The modA/tupA/wtpA gene encodes a periplasmic molybdate/tungstate-binding protein (protein A) which constitutes the first selection gate from which cells should differentiate between Mo and W. The ModA, WtpA, and TupA proteins differ in their binding affinity for molybdate versus tungstate, primary sequence and oxoanion coordination chemistry. The present work reports the 1.40 Å crystal structure of the recombinant apo-form of TupA protein from the sulfate reducing bacteria Desulfovibro alaskensis G20 (DaG20 TupA) together with the biochemical characterization of three variants: R118K, R118E and R118Q. X-ray crystallography and SAXS, reveals that TupA architecture has a common feature with other substrate binding proteins, which is the existence of two separate lobes.

TupA is a globular protein with approximate dimensions of 55.7 × 34.5 × 23.8 Å. The protein has a butterfly shape with a central beta strand (T77-P89) that supports two lobes (lobe A: A2-R76 and Y201-E251; lobe B: A91-Q200). The central beta strand is hydrogen bonded to three beta strands of each of the lobes forming two 4-stranded beta sheets. The TupA metal binding site is located in a central cleft assembled by the two lobes. In DaG20 TupA, the cleft is decorated with positively charged residues as seen by the electrostatic surface potential calculations. The pronounced positive environment of the pocket must be an advantage to enable capture of the oxyanion, even when the extracellular concentration is low. Moreover, one chloride anion, arising from the crystallization conditions, was found at 3.8 Å from R118, indicating the propensity of the pocket to attract negatively charged ions. In this GsTupA-W6+ holo form, the central cleft volume (363.9 Å3) is four times smaller than the apo form of DaG20 TupA here reported (1480 Å3). The apo-form model was created by refining the initial BUNCH model with the SREFLEX program. This approach revealed a slight opening of the lobes (RMSD of 1.5 Å for 274 Cα atoms) yielding an excellent agreement to the TupA SAXS data measured in the absence of tungstate or molybdate (χ2 = 1.0). The SAXS data corroborate the hypothesis that DaG20 TupA is a flexible protein that is able to adopt a loose conformation in the free form but, when binding to molybdate or tungstate, switches to a more compact fold.

> MAHHHHHHVDDDDKMLEVLFQGPEAPVLMMATTTSTDNTGLLDDLAPQFTKDTGIELRWTAVGTGKALKMGENCDVDILLVHAPAAEKAFVDAGFGTARTQLMYNDFVIIGPAADPAGVKGMTVAAALGKIAADNAVFVSRGDNSGTHKMEKSLWKQIEGPSPEKEAWYVQTGQGMLRTINVAAEKGGYTMTDRGTYIKYEASMDGNPPLKILVEGDKILFNQYSAIPVNPAHCPKVKKDLADKFVNWMASPATQKTIGDFKLMGKALFTPNAE> HHHHHHMAITKPLLAATLENIEDVQFPCLATPKIDGIRSVKQTQMLSRTFKPIRNSVMNRLLTELLPEGSDGEISIEGATFQDTTSAVMTGHKMYNAKFSYYWFDYVTDDPLKKYIDRVEDMKNYITVHPHILEHAQVKIIPLIP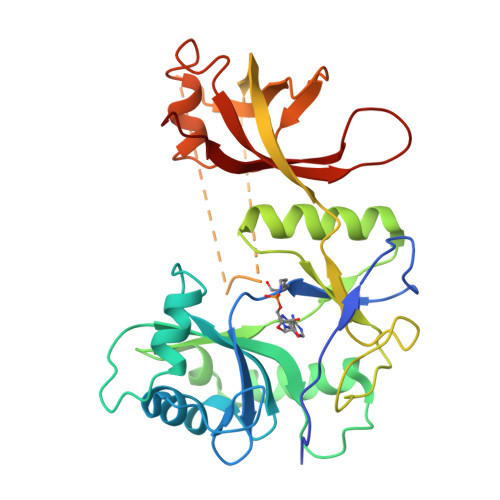VEINNITELLQYERDVLSKGFEGVMIRKPDGKYKFGRSTLKEGILLKMKQFKDAEATIISMTALFKNTNTKTKDNFGYSKRSTHKSGKVEEDVMGSIEVDYDGVVFSIGTGFDADQRRDFWQNKESYIGKMVKFKYFEMGSKDCPRFPVFIGIRHEEDR1H-indole-6-carbonitrile | C9 H6 N2 | 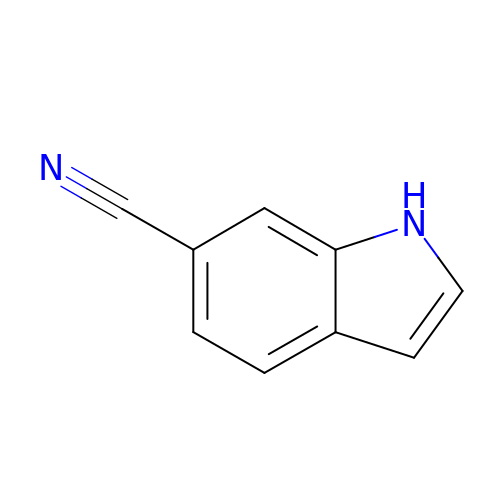SZSZDBFJCQKTRG-UHFFFAOYSA-N The mechanistic target of rapamycin complex 1 (mTORC1) integrates growth factor (GF) and nutrient signals to stimulate anabolic processes connected to cell growth and inhibit catabolic processes such as autophagy. Direct binding of RHEB–GTP to the mTOR kinase subunit of mTORC1 allosterically activates the kinase by inducing a large-scale conformational change. Despite the fact that the receptor–PI3K–AKT signalling pathway originates at the plasma membrane, RHEB signalling to mTORC1 occurs exclusively on the cytosolic face of lysosomes. mTORC1 is recruited to lysosomes by the RAS-related GTP-binding (RAG) GTPases RAGA–RAGD under amino acid-replete conditions. Here we reconstituted mTORC1 activation on membranes by RHEB, RAGs and Ragulator.

Using symmetry expansion and particle subtraction to remove RAPTOR–RAG–Ragulator, we performed 3D classification on the subpopulation that does not contain extra RAG–Ragulator copies and identified two distinct conformations of the mTOR–RHEB–MLST8 subcomplex. The final resolutions of the intermediate and fully active states were 3.61 Å and 3.16 Å, respectively. The M-HEAT domain of the active state moved closer to the N-HEAT domain than it did with the intermediate state, with an average distance of about 5 Å. The FAT and kinase domains of the fully active state moved about 5–7 Å towards RHEB compared with those in the intermediate state. The mTOR–RHEB interaction is largely maintained in both intermediate and fully active states; however, the residues Met1255 and Lys1256 of the FAT domain of mTOR are disordered in the intermediate state but engaged with RHEB in the active state. In the mTOR intermediate state, Tyr35 in the switch I region of RHEB flips to the opposite side and is disengaged from the nucleotide, whereas, in the mTOR fully active state, the switch I region of RHEB adopts the canonical conformation of the RHEB–GTP-bound state. The FAT domain of mTOR is more engaged with the C-lobe in the fully active state than in the intermediate state. The established electrostatic interactions between residues Glu1581 and Gln1355 in the FAT domain and between residues Arg1585 of the FAT domain and Glu2311 of the C-lobe in the fully active state indicate direct communication between the FAT domain and the kinase domain to promote the active state. In the fully active state, the ATP molecule was positioned 1.5 Å closer to the catalytic residues in the C-lobe than in the soluble mTORC1–RHEB structure, aligning more closely with other atypical serine–threonine kinases in the phosphatidylinositol-3-kinase-related kinase (PIKK) family in their active states. Finally, the mTOR–membrane-interacting site is only seen to dock in the fully active state (4), suggesting that this interaction is involved in finally reaching the highest level of activation.

> MLGTGPAAATTAATTSSNVSVLQQFASGLKSRNEETRAKAAKELQHYVTMELREMSQEESTRFYDQLNHHIFELVSSSDANERKGGILAIASLIGVEGGNATRIGRFANYLRNLLPSNDPVVMEMASKAIGRLAMAGDTFTAEYVEFEVKRALEWLGADRNEGRRHAAVLVLRELAISVPTFFFQQVQPFFDNIFVAVWDPKQAIREGAVAALRACLILTTQREPKEMQKPQWYRHTFEEAEKGFDETLAKEKGMNRDDRIHGALLILNELVRISSMEGERLREEMEEITQQQLVHDKYCKDLMGFGTKPRHITPFTSFQAVQPQQSNALVGLLGYSSHQGLMGFGTSPSPAKSTLVESRCCRDLMEEKFDQVCQWVLKCRNSKNSLIQMTILNLLPRLAAFRPSAFTDTQYLQDTMNHVLSCVKKEKERTAAFQALGLLSVAVRSEFKVYLPRVLDIIRAALPPKDFAHKRQKAMQVDATVFTCISMLARAMGPGIQQDIKELLEPMLAVGLSPALTAVLYDLSRQIPQLKKDIQDGLLKMLSLVLMHKPLRHPGMPKGLAHQLASPGLTTLPEASDVGSITLALRTLGSFEFEGHSLTQFVRHCADHFLNSEHKEIRMEAARTCSRLLTPSIHLISGHAHVVSQTAVQVVADVLSKLLVVGITDPDPDIRYCVLASLDERFDAHLAQAENLQALFVALNDQVFEIRELAICTVGRLSSMNPAFVMPFLRKMLIQILTELEHSGIGRIKEQSARMLGHLVSNAPRLIRPYMEPILKALILKLKDPDPDPNPGVINNVLATIGELAQVSGLEMRKWVDELFIIIMDMLQDSSLLAKRQVALWTLGQLVASTGYVVEPYRKYPTLLEVLLNFLKTEQNQGTRREAIRVLGLLGALDPYKHKVNIGMIDQSRDASAVSLSESKSSQDSSDYSTSEMLVNMGNLPLDEFYPAVSMVALMRIFRDQSLSHHHTMVVQAITFIFKSLGLKCVQFLPQVMPTFLNVIRVCDGAIREFLFQQLGMLVSFVKSHIRPYMDEIVTLMREFWVMNTSIQSTIILLIEQIVVALGGEFKLYLPQLIPHMLRVFMHDNSPGRIVSIKLLAAIQLFGANLDDYLHLLLPPIVKLFDAPEAPLPSRKAALETVDRLTESLDFTDYASRIIHPIVRTLDQSPELRSTAMDTLSSLVFQLGKKYQIFIPMVNKVLVRHRINHQRYDVLICRIVKGYTLADEEEDPLIYQHRMLRSGQGDALASGPVETGPMKKLHVSTINLQKAWGAARRVSKDDWLEWLRRLSLELLKDSSSPSLRSCWALAQAYNPMARDLFNAAFVSCWSELNEDQQDELIRSIELALTSQDIAEVTQTLLNLAEFMEHSDKGPLPLRDDNGIVLLGERAAKCRAYAKALHYKELEFQKGPTPAILESLISINNKLQQPEAAAGVLEYAMKHFGELEIQATWYEKLHEWEDALVAYDKKMDTNKDDPELMLGRMRCLEALGEWGQLHQQCCEKWTLVNDETQAKMARMAAAAAWGLGQWDSMEEYTCMIPRDTHDGAFYRAVLALHQDLFSLAQQCIDKARDLLDAELTAMAGESYSRAYGAMVSCHMLSELEEVIQYKLVPERREIIRQIWWERLQGCQRIVEDWQKILMVRSLVVSPHEDMRTWLKYASLCGKSGRLALAHKTLVLLLGVDPSRQLDHPLPTVHPQVTYAYMKNMWKSARKIDAFQHMQHFVQTMQQQAQHAIATEDQQHKQELHKLMARCFLKLGEWQLNLQGINESTIPKVLQYYSAATEHDRSWYKAWHAWAVMNFEAVLHYKHQNQARDEKKKLRHASGANITNATTAATTAATATTTASTEGSNSESEAESTENSPTPSPLQKKVTEDLSKTLLMYTVPAVQGFFRSISLSRGNNLQDTLRVLTLWFDYGHWPDVNEALVEGVKAIQIDTWLQVIPQLIARIDTPRPLVGRLIHQLLTDIGRYHPQALIYPLTVASKSTTTARHNAANKILKNMCEHSNTLVQQAMMVSEELIRVAILWHEMWHEGLEEASRLYFGERNVKGMFEVLEPLHAMMERGPQTLKETSFNQAYGRDLMEAQEWCRKYMKSGNVKDLTQAWDLYYHVFRRISKQLPQLTSLELQYVSPKLLMCRDLELAVPGTYDPNQPIIRIQSIAPSLQVITSKQRPRKLTLMGSNGHEFVFLLKGHEDLRQDERVMQLFGLVNTLLANDPTSLRKNLSIQRYAVIPLSTNSGLIGWVPHCDTLHALIRDYREKKKILLNIEHRIMLRMAPDYDHLTLMQKVEVFEHAVNNTAGDDLAKLLWLKSPSSEVWFDRRTNYTRSLAVMSMVGYILGLGDRHPSNLMLDRLSGKILHIDFGDCFEVAMTREKFPEKIPFRLTRMLTNAMEVTGLDGNYRITCHTVMEVLREHKDSVMAVLEAFVYDPLLNWRLMDTNTKGNKRSRTRTDSYSAGQSVEILDGVELGEPAHKKTGTTVPESIHSFIGDGLVKPEALNKKAIQIINRVRDKLTGRDFSHDDTLDVPTQVELLIKQATSHENLCQCYIGWCPFW;> MNTSPGTVGSDPVILATAGYDHTVRFWQAHSGICTRTVQHQDSQVNALEVTPDRSMIAAAGYQHIRMYDLNSNNPNPIISYDGVNKNIASVGFHEDGRWMYTGGEDCTARIWDLRSRNLQCQRIFQVNAPINCVCLHPNQAELIVGDQSGAIHIWDLKTDHNEQLIPEPEVSITSAHIDPDASYMAAVNSTGNCYVWNLTGGIGDEVTQLIPKTKIPAHTRYALQCRFSPDSTLLATCSADQTCKIWRTSNFSLMTELSIKSGNPGESSRGWMWGCAFSGDSQYIVTASSDNLARLWCVETGEIKREYGGHQKAVVCLAFNDSVLG;> MPQSKSRKIAILGYRSVGKSSLTIQFVEGQFVDSYDPTIENTFTKLITVNGQEYHLQLVDTAGQDEYSIFPQTYSIDINGYILVYSVTSIKSFEVIKVIHGKLLDMVGKVQIPIMLVGNKKDLHMERVISYEEGKALAESWNAAFLESSAKENQTAVDVFRRIILEAEKMDGAASQGKSSCSVM>[2x]ASMKIVVITEKPFAENAVKGIREILEKAGHEVVMIEKYKKKEDVIERIKDADGVIVRSDKIDEEIIKAGEKVKIIVRAGAGYDNIDIEACNQGKIVVMNTPGQNRNGVAELCIGMMIFGFRKGFKEGKGRELKDKTLGICGCGYVGKRVKEIAEGIGMKIKVYDPFITTENQVKKIEELFEECQVISLHLPLTKETKGKIGYELIKKLPYGGM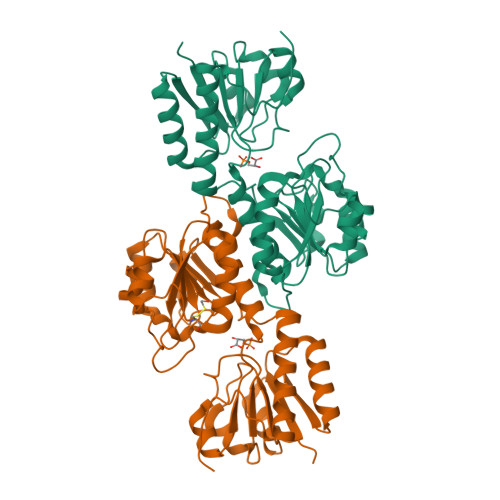ICNTARKEIIDEEGLIRIMREREDLIYITDVAPTSKVFNNEFKGRFFATPIKIGAETEESNINAGMAAASQICDFFTNGTVKFQVNKFLEHHHHHH>[10x]DEIKIVKYPDPILRRRSEVTNFDDNLKRVVRKMFDIMYE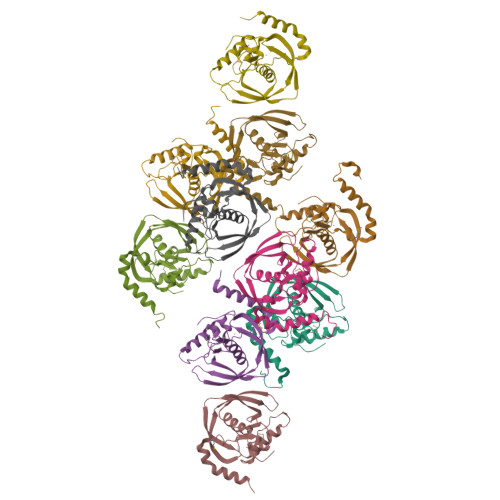SKGIGLSAPQVNISKRIIVWNALYEKRKEENERIFINPSIVEQSLVKLKLIEGCLSFGIEGKVERPSIVSISYYDINGYKHLKILKGIHSRIFQHEFDHLNGTLFIDKMTQVDKKKVRPKLNELIRDYKATHSEEPLEHHHHHH2-[3-(3-methoxy-4-nitrophenyl)-11-oxo-10,11-dihydro-5H-dibenzo[b,e][1,4]diazepin-8-yl]-N,N-dimethylacetamide 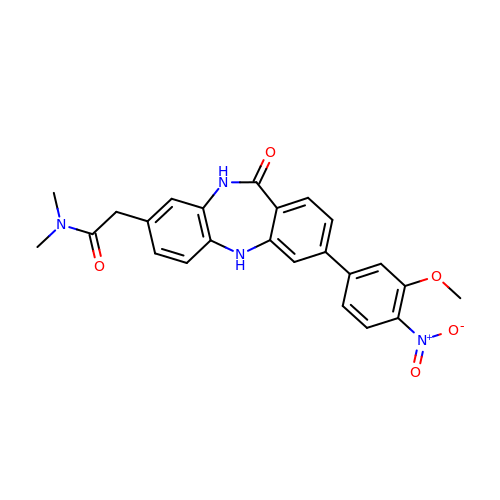| C24 H22 N4 O5 | FDMSWGUJFDPKLS-UHFFFAOYSA-N Our findings provide insight into the mechanism underlying the activity of MTHFD from B. mori and potentially other insects and may therefore facilitate the development of inhibitors specific to MTHFD as insecticides.

The bmMTHFD structure was determined at a resolution of 1.75 Å by X‐ray crystallography. Site‐directed mutagenesis indicated that the amino acid residue Tyr49 contributed to its catalytic activity.

>MARILDGKALAMEIKKELKQKIAQWVSLGNRAPTIRCIIVGDDPASHTYVRNKVEAAKFVGIDALTINRDSDITEEQLLSEIQNLNEDNSVDGILVQLPVPDTINERRVCDAIAPEKDIDGFHIINIGRLCVDLPTIVPATALAVVEMLKRFNIDTFGRNAVVIGRSKNVGMPIAMMLHSDKRHESGLGMDATVTICHRYTPKDKLEAYCRNADIIITATGLPKLIKADMVKPGATIIDVGITTRTDENGKSRLVGDVDYEEVSKIAGAITPVPGGVGPMTVAMLMHNTFQAAQSQANKSN[2x]The tenovins are a frequently studied class of compounds capable of inhibiting sirtuin activity, which is thought to result in increased acetylation and protection of the tumor suppressor p53 from degradation. In this study, we present two additional mechanisms by which tenovins are able to activate p53 and kill tumor cells in culture. These mechanisms are the inhibition of a key enzyme of the de novo pyrimidine synthesis pathway, dihydroorotate dehydrogenase (DHODH), and the blockage of uridine transport into cells. The blockage of DHODH by another chemical class adds to our previous findings that DHODH is a frequently hit target of small molecules.

We used an enzyme activity assay to assess the effect of tenovins on DHODH enzymatic activity. This assay revealed that a number of tenovin analogues are capable of inhibiting DHODH (IC50 shown in Fig. 1B and Fig. S2). We finally obtained a crystal structure of tenovin 6 co-crystallized with DHODH. This crystal structure demonstrated that the tenovins bind in the same pocket as our previously published compound, HZ05 (16) as well as brequinar and teriflunomide. Based on the crystal structure of tenovin 6 co-crystallized with DHODH, we decided to model the potential interactions of the tenovins with DHODH to examine the energetic favorability of the interaction. Our structural models were constructed using the apo-structure of DHODH and refined using extensive molecular dynamics (MD) simulations. The models suggest that tenovin 1 possesses the same predicted interaction at Gln-46 as tenovin 6 and that the reversed amide present in tenovin 39, tenovin 39OH, tenovin 50, and tenovin 50OH is not favored. Now it has been established that tenovin 6 has two additional mechanisms of action, DHODH inhibition and blockage of uridine uptake, along with the previously established targets SirT1 and SirT2 (11) as well as blockage of autophagic flux.

> MATGDERFYAEHLMPTLQGLLDPESAHRLAVRFTSLGLLPRARFQDSDMLEVRVLGHKFRNPVGIAAGFDKHGEAVDGLYKMGFGFVEIGSVTPKPQEGNPRPRVFRLPEDQAVINRYGFNSHGLSVVEHRLRARQQKQAKLTEDGLPLGVNLGKNKTSVDAAEDYAEGVRVLGPLADYLVVNVSSPNTAGLRSLQGKAELRRLLTKVLQERDGLRRVHRPAVLVKIAPDLTSQDKEDIASVVKELGIDGLIVTNTTVSRPAGLQGALRSETGGLSGKPLRDLSTQTIREMYALTQGRVPIIGVGGVSSGQDALEKIRAGASLVQLYTALTFWGPPVVGKVKRELEALLKEQGFGGVTDAIGADHRR> MGSSNTVTSAVKTQYVEIESVMGFYFNTEDKFDTAQIKKAVLHTVYNEGYTGDDGVAVVLREYESEPVDITAELTFGDATPANTYKAVENKFDYEIPVYYNNATLKDAEGNDATVTVYIGLKGDTDLNNIVDGRDATATLTYYAATSTDGKDATTVALSPSTLVGGNPESVYDDFSAFLSDVKVDAGKELTRFAKKAERLIDGRDASSILTFYTKSSVDQYKDMAANEPNKLW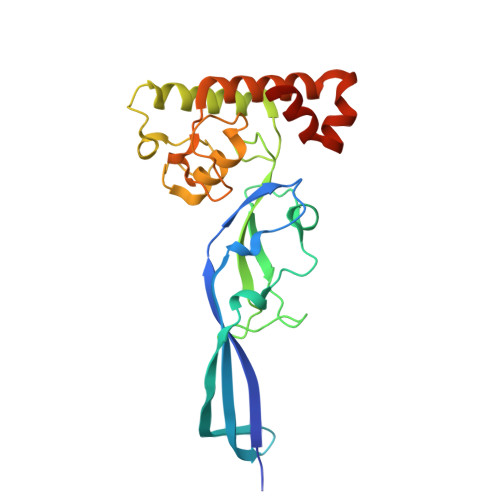DIVTADAEEE> AIAFEHVTYTYQAGTPMAH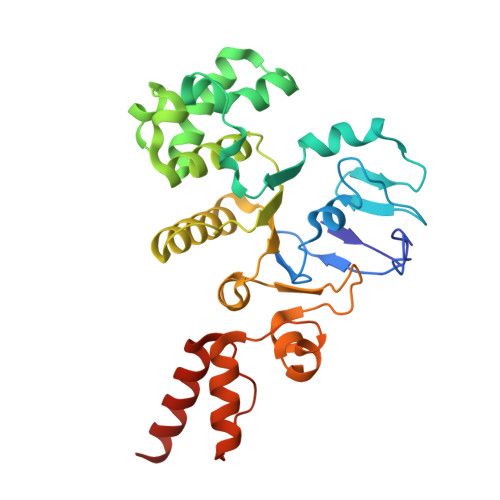TALTDVSLTVPDRGYLAIIGHTGSGKSTLIQQLNALLKPTSGTIKIDEFTITPETTNAALKPLRQHVGMVFQFPENQLFEETVRQDIAFGPKNFGMADADALALADEMLTTVGLDQSYAERSPFELSGGQMRRVAIAGVLAMQPKVLVLDEPTAGLDPQGRQEMMRLFARLHQEQGLTIVLVTHQMEDVAQYAEQVAVMHEGRLMKFGTPADVFSNREWLQDHQLDVPQAAQFARRLRDRGLTFPKQPLTADQLADYLAQQWAQRGADHV2-fluoro-4-{[(1R)-6-methoxy-1-methyl-1-{2-oxo-2-[(1,3-thiazol-2-yl)amino]ethyl}-1,2,3,4-tetrahydroisoquinolin-7-yl]oxy}benzoic 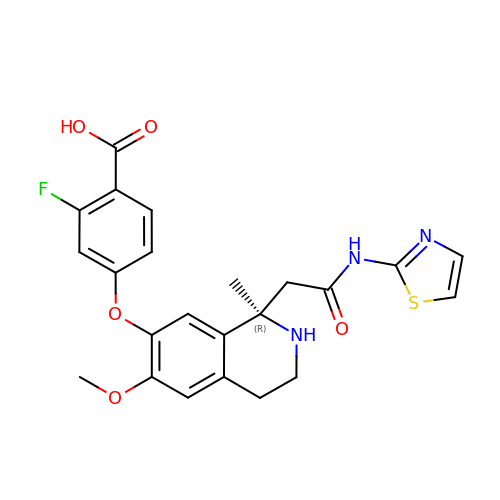acid | C23 H22 F N3 O5 S | PZYUALDJGJBZEM-HSZRJFAPSA-N> MLQVDIGSTSGKAGSVVSVPITFTNVPKSGIYALSFRTNFDPQKVTVASIDAGSLIENASDFTTYYNNENGFASMTFEA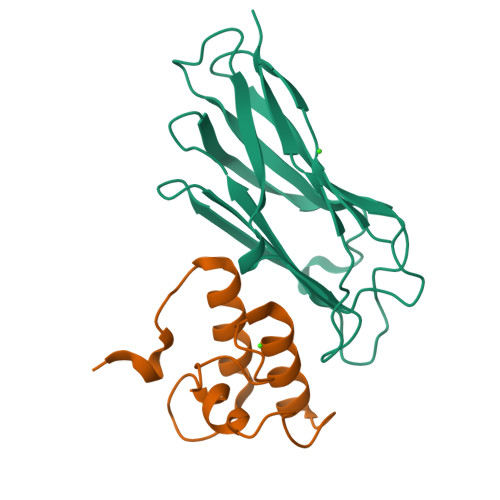PVDRARIIDSDGVFATINFKVSDSAKVGELYNITTNSAYTSFYYSGTDEIKNVVYNDGKIEVIALEHHHHHH;> KFIYGDVDGNGSVRINDAVLIRDYVLGKINEFPYEYGMLAADVDGNGSIKSIDAVLVRDYVLGKIFLFPVEEKEE>MYGYDGKVLRINLKERTCKSENLDLDKAKKFIGCRGLGVKTLFDEIDPKIDALSPENKFIIVTGPLTGAPVPTSGRFMVVTKAPLTGTIGISNSGGKWGVDLKKAGWDMIIVEDKADSPVYIEIVDDKVEIKDASQLWGKVTSETTKELEKITENKSKVLCIGPAGERLSLMAAVMNDVDRTAARGGVGAVMGSKNLKAITVKGTGKIALADKEKVKKVSVEKITTLKNDPVAGQGMPTYGTAILVNIINENGVHPVKNFQESYTNQADKISGETLTANQLVRKNPCYSCPIGCGRWVRLKDGTECGGPEYETLWCFGSDCGSYDLDAINEANMLCNEYGIDTITCGATIAAAMELYQRGYIKDEEIAGDNLSLKWGDTESMIGWIKRMVYSEGFGAKMTNGSYRLCEGYGAPEYSMTVKKQEIPAYDPRGIQGHGITYAVNNRGGCHIKGYMINPEILGYPEKLDRFALDGKAAYAKLFHDLTAVIDSLGLCIFTTFGLGIQDYVDMYNAVVGESTYDADSLLEAGDRIWTLEKLFNLAAGIDSSQDTLPKRLLEEPIPDGPSKGEVHRLDVLLPEYYSVRGWSKEGIPTEETLKKLGLDEYIGKF[2x]

Here, we experimentally validated that ethanol production is initiated through a tungsten-dependent aldehyde:ferredoxin oxidoreductase (AFOR), which reduces acetate to acetaldehyde. All these oxidoreductases contain two metallocofactors: a [4Fe–4S] cluster and a W-containing bis-pyranopterindithiolene cofactor (simplified here as tungstopterin). To solve this metabolic riddle, we characterized the native AFOR of C. autoethanogenum (CaAFOR) by X-ray crystallography, biochemistry and enzymology. By performing the reversible conversion of different aldehydes into acids, AFORs are environmentally and biotechnologically relevant enzymes, putatively valuable for synthetic biology.

The crystal structure of holo AFOR, refined to 1.59-Å resolution, and its biochemical characterization provide new insights into the cofactor chemistry and the specificities of this enzyme, fundamental to sustainable biofuel production. X-ray fluorescence measurement on protein crystals confirmed the presence of W in CaAFOR and the structure was experimentally solved by single-wavelength anomalous diffraction at the W L3 edge. The crystal asymmetric unit contains two CaAFORs, which have too weak of an interaction to be stable in solution, confirming the monomeric state, unlike structurally characterized homologs. However, the overall monomeric structure is highly similar to the structures of the homologs, the AFOR from P. furiosus being the closest. The tungstopterin cofactor of CaAFOR exhibits a canonical composition with two pyranopterindithiolene groups, stabilized in a ‘bent conformation’ by the coordination of the flanking phosphates with a Mg atom. The W atom is coordinated by the dithiolene groups from each pterin and by two atoms modeled as oxygen according to the electron density. The W–O distances in the CaAFOR structure are, however, substantially longer (around 2.2 Å) than the W=O double bond modeled in the structure from A. aromaticum (1.74–1.75 Å) or detected by EXAFS spectroscopy (1.74 Å). On the basis of the observed distance, the ligands were modeled as hydroxo rather than oxo groups. One of the hydroxyl groups establishes short hydrogen bonds with the perfectly conserved glutamate (E312) and histidine (H448), a position that should be occupied by the acetaldehyde and acetate molecules and reaction intermediates. To evaluate the CaAFOR redox states observed in the crystal structure, we incubated the as-isolated protein with an excess of BV2+ and barely detected a reduction of the artificial electron acceptor (with an estimated 0.1 mol of electrons per mol of CaAFOR). This suggests that CaAFOR was crystallized mostly in a fully oxidized W(VI) state.> MGHSSSDPVYPCGICTNEVNDDQDAILCEASCQKWFHRICTGMTETAYGLLTA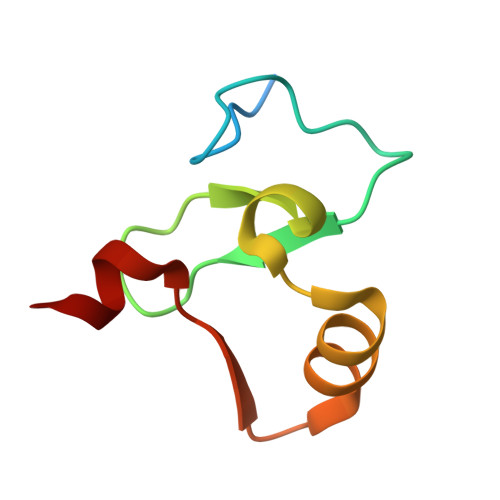EASAVWGCDTCMAD> GFSTMAQQSGGGLTRGSFPEGFVFGTASAAYQYEGAVKEDGRGQTIWDTFAHTFGKITDFSNADVAVDQYHRFEEDIQLMADMGMDAYRFSIAWSRIYPNGVGQVNQAGIDHYNKLIDALLAKGIQPYVTLYHWDLPQALEDKYKGWLDRQIVDDFAAYAETCFREFGDRVKHWITLNQPHTVAIQGYDAGLQAPGRCSVLLHLYCKAGNSGTEPYVVAHHFILAHAAAASIYRTKYKATQNGQLGIAFDVMWFEPMSNTTIDIEAAKRAQEFQLGWFADPFFFGDYPATMRARVGERLPRFTADEAAVVKGALDFVGINHYTTYYTRHNNTNIIGTLLNNTLADTGTVSLPFKNGKPIGDRANSIWLYIVPRGMRSLMNYVKERYNSPPVYITENGMDDSNNPFISIKDALKDSKRIKYHNDY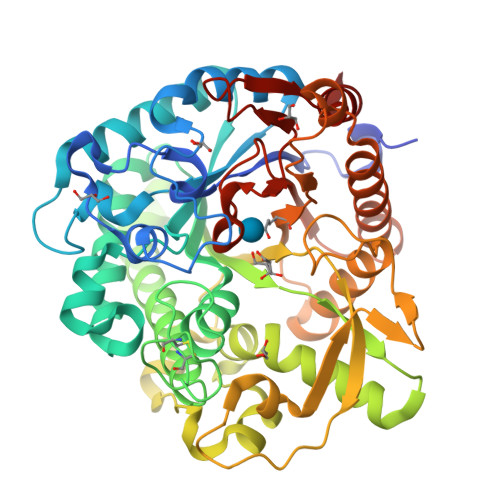LTNLAASIKEDGCDVRGYFAWSLLDNWEWAAGYSSRFGLYFVDYKDNLKRYPKNSVQWFKALLKT> EGFKANLSLLRRPGEKTYTQRCRLFVGNLPADITEDEFKRLFAKYGEPGEVFINKGKGFGFI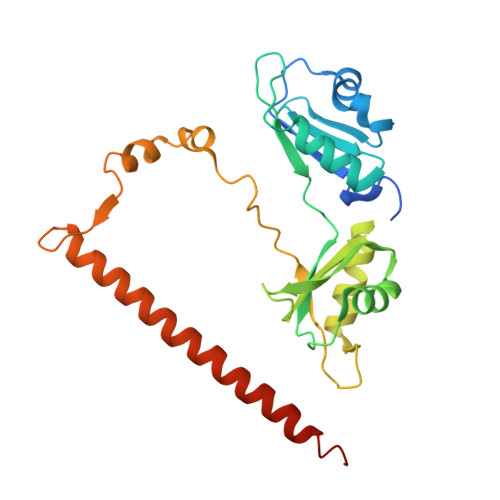KLESRALAEIAKAELDDTPMRGRQLRVRFATHAAALSVRNLSPYVSNELLEEAFSQFGPIERAVVIVDDRGRSTGKGIVEFASKPAARKAFERCSEGVFLLTTTPRPVIVEPLEQLDDEDGLPEKLAQKNPMYQKERETPPRFAQHGTFEYEYSQRWKSLDEMEKQQREQVEKNMKDAKDKLESEMEDAYHEHQANLL> GPLGSKRVIVIGGALAETAFALGGAETPRYRLVGADTTCTYPDAAKRLPKVGYQRALSAEGLLSLRPDLVLASAEAGPPTAIAQVKGAGVTVTTFDERHDVESVRAKI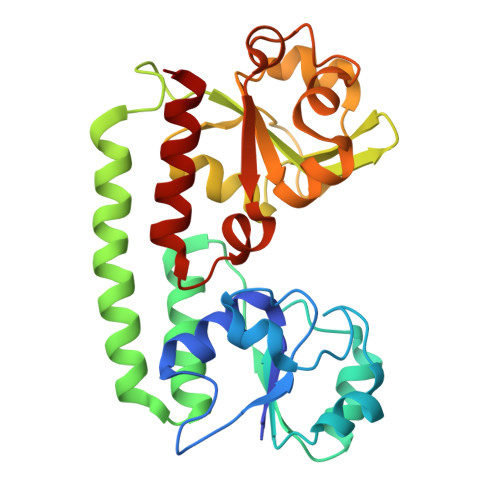TGVAQALDVRDAGAALLQRFDRDWQAARDAVAARVPGGAQPPRVLFVLNHTGTQALVAGQRTAADAMIRYAGARNAMQGFDHYKPLTTEALAAAAPDVVLISDEGLAAVGGHAALLATPGFGATPAGRARRVVSLDALFLLGFGPRLPLAVTTLHRRLSDALA>GPMVSLAQVRGALCGALLGDCMGAEFEGSDAVELPDVLEFVRLLEKEKKAGTLFYTDDTAMTRAVIQSLIAKPDFDEVDMAKRFAEEYKKEPTRGYGAGVVQVFKKLLSPKYSDVFQPAREQFDGKGSYGNGGAMRVASIALAYPNIQDVIKFARRSAQLTHASPLGYNGAILQALAVHFALQGELKRDTFLEQLIGEMERIEGGEMSASDAGEHDRPNEVKLPFCSRLKKIKEFLASSNVPKADIVDELGHGIAALESVPTAIYSFLHCMESDPDIPDLYNNLQRTIIYSI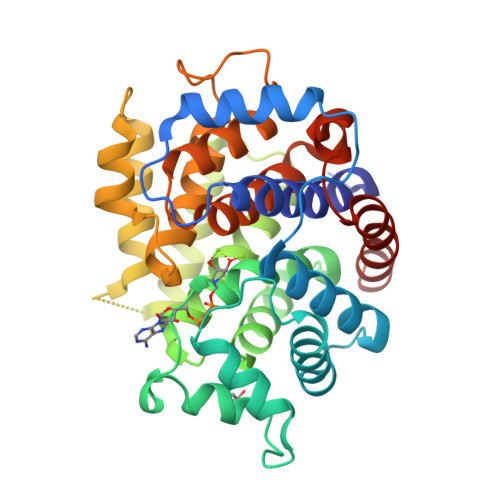SLGGDTDTIATMAGAIAGAYYGMDQVTPSWKRSCEAIVETEESAVKLYELYCKQLKTP[2x]ethyl 5-hydroxy-4-[(4-methylpiperidin-1-yl)methyl]-2-phenyl-1-benzofuran-3-carboxylate 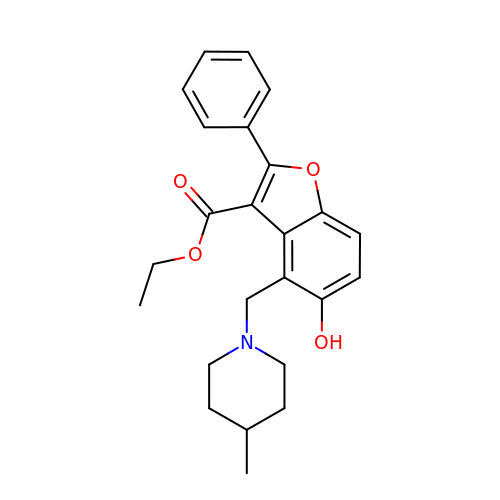| C24 H27 N O4 | YDARBKORYFGQMH-UHFFFAOYSA-N> VAFGADAAKTTQEKFDALKEAGVFSAYPGTTDAKLGQDMTRAEFAKVLVKLFGLKEIHGQYSYKDKNYDAKNWAAPFIEAVTAEGLMQAKDLTKKIFDFNGKITVEEASKTLVTALKLEPVKDAQNKATDWAKGYFEAAVNAGLFSKDANPKANATRAQLVEAAFAADEMSKGSGSHHHHHH

Prokaryotic cell envelopes often include proteinaceous surface (S-) layers composed of self-assembling subunits in porous two-dimensional crystalline lattices. S-layer anchoring is best characterized for Gram-positive bacteria, where S-layer proteins non-covalently attach to the PG layer via species- and strain-specific non-classical secondary cell wall polymers (SCWPs). SpaA possesses three consecutive SLH domains near its N-terminus, followed by a large C-terminal region presumed to harbor the self-assembling domain(s). The crystal structures and binding analyses presented here of P. alvei SpaASLH, SpaASLH/G109A, and SpaASLH/G46A/G109A with synthetic SCWP fragments provide novel insights into the functional contributions of many conserved SLH domain residues, including SLH-Trp13, SLH-Gly29, and SLH-Arg43, which precisely interlock from three different SLH domains to generate two active binding sites.

To demonstrate conclusively the significance of the conserved SLH-Gly29 and the backbone flip for SCWP binding, we created a double mutant SpaASLH/G46A/G109A for binding and structural analysis. As expected, this mutant displays no detectable binding to 4,6-Pyr-β-d-ManNAcOMe by ITC. The crystal structure of SpaASLH/G46A/G109A displays the same groove conformations as wt SpaASLH and unliganded SpaASLH/G109A, with G2 narrower than G1. Residues 46–55 in G1 are in a similar conformation as in the unliganded SpaASLH/G109A structure, but with a slight widening of the loop to accommodate the Gly46Ala mutation. Despite the lack of binding detected by ITC, ligand is again observed bound in the G2 pocket, albeit with Gln108 and Ala109 in the unliganded backbone conformation (i.e., not flipped). The monosaccharide is bound with the same interactions as observed for wt SpaASLH, except that there is no hydrogen bond between the pyruvyl carboxyl oxygen and Gly109 nitrogen, but instead there is a minor movement of ligand away from the Gln108 carbonyl that results in a less ideal bidentate interaction with Arg61. The observation of bound ligand in the crystal structure despite no binding being detected by ITC, similar to the observation of 2:1 binding in the wt SpaASLH crystal structure despite 1:1 binding measured by ITC, indicates again that affinity is markedly increased in the crystal context.> MGSSHHHHHHTGGTHPAVRVADLLQHINQMKTAEGYGFKQEYESFFEGWDATKKKDKVKGSRQEPMPAYDRHRVKL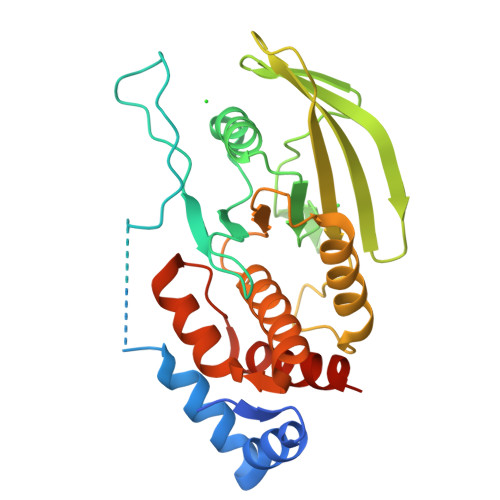HPMLGDPSADYINANYIDGYHRSNHFIATQGPKPEMVYDFWRMVWQEHCSSIVMITKLVEVGRVKCSRYWPEDSDTYGDIKIMLVKTETLAEYVVRTFALERRGYSARHEVRQFHFTAWPEHGVPYHATGLLAFIRRVKASTPPDAGPIVIHCSAGTGRTGCYIVLDVMLDMAECEGVVDIYNCVKTLCSRRVNMIQTEEQYIFIHDAILEACLCGETTIP Two racemic crystal structures of the DNA sequence d(CCCGGG) are described which were found to fold into A-form DNA. This form differs from the Z-form DNA conformation adopted by the chiral equivalent in the solid state, suggesting that the use of racemates may also favour the emergence of new conformations. Importantly, the racemic mixture forms interactions in the solid state that differ from the chiral equivalent (including the formation of racemic pseudo-helices), suggesting that the use of racemic DNA mixtures could provide new possibilities for the design of precise self-assembled nanomaterials and nanostructures.

We next turned to a sparse-matrix crystallization screening approach, which successfully identified two related conditions suitable for crystal growth. X-ray diffraction analyses of the two crystal forms indicated that the crystals belonged to the achiral space groups and P21/n, in line with previous findings describing the tendency of racemic DNA mixtures to form racemic crystals rather than conglomerates. Both crystal structures were solved by molecular replacement, with the resulting refined electron-density maps being of sufficiently high quality to allow the chirality of the DNA strands to be unambiguously determined. Analysis of the duplex geometry reveals parameters that are all in line with expectations for A-DNA, namely a rise per residue of ∼2.8–3.0 Å, a base-pair inclination of ∼9–13° and a preference for C3′-endo sugar puckers. To our knowledge, this is the first report of a racemic crystal structure of A-form DNA. The racemic A-form duplex crystal structures that we report here therefore add to the array of conformations adopted by this DNA sequence, providing further evidence of the considerable structural polymorphism of this motif. Perhaps paradoxically, despite this apparent structural polymorphism, the five independent A-type duplexes present within these two crystal structures reveal a remarkable degree of structural similarity, as indicated by structural alignments, despite the differences in space group and crystal packing. Heterochiral pseudo-continuous helices are helices in which d-DNA duplexes and l-DNA duplexes stack end-to-end in an alternating manner, with an inversion of the helix handedness at every helix–helix contact. Thus, the racemic d/l-d(CCCGGG) sequence studied here reveals packing interactions that have not previously been observed, suggesting that racemic mixtures of DNA sequences may generate assemblies and higher-order structures that are not accessible to equivalent enantiopure systems.

>CCCGGG[4x]>CCCGACUUAAGU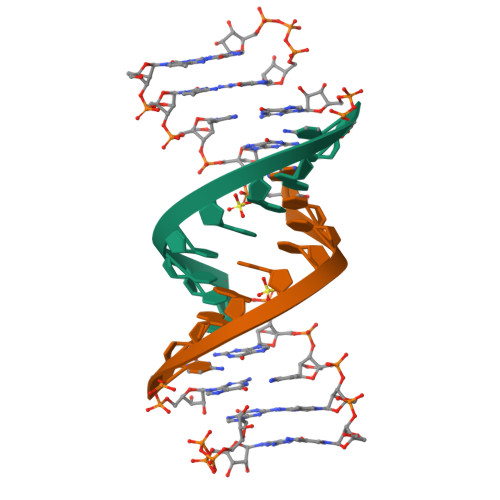CG[2x]(S)-2-AMINO-5-(2-MERCAPTOACETIMIDAMIDO)PENTANOIC ACID | C7 H15 N3 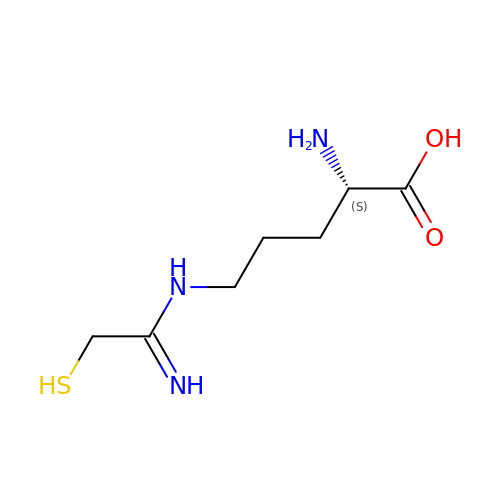O2 S | ROQCTZSRBCTHGN-YFKPBYRVSA-N>GSPSLKIAPANADFAFRFYYLIASETPGKNIFFSPLSISAAYAMLSLGACSHSRSQILEGLGFNLTELSESDVHRGFQHLLHTLNLPGHGLETRVGSALFLSHNLKFLAKFLNDTMAVYEAKLFHTNFYDTVGTIQLINDHVKKETRGKIVDLVSELKKDVLMVLVNYIYFKALWEKPFISSRTTPKDFYVDENTTVRVPMMLQDQEHHWYLHDRYLPCSVLRMDYKGDATVFFILPNQGKMREIEEVLTPEMLMRWNNLLRKRNFYKKLELHLPKFSISGSYVLDQILPRLGFTDLFSKWADLSGITKQQKLEASKSFHKA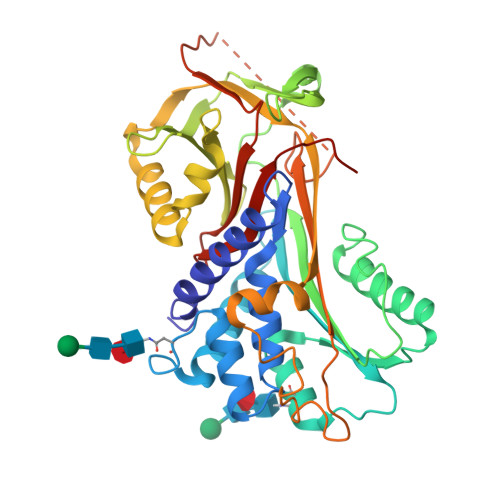TLDVDEAGTEAAAATSFAIKFFSAQTNRHILRFNRPFLVVIFSTSTQSVLFLGKVVDPTKPHHHHHH[2x]> GSHMGFRWKLAHFRYLCQSNALPSHVKINVSRQTLFEDSFQQIMALKPYDLRRRLYVIFRGEEGLDYGGLAREWFFLLSHEVLNPMYCLFEYAGKNNYCLQINPASTINPDHLSYFCFIGRFIAMALFHGKFIDTGFSLPFYKRMLSKKLTIKDLESIDTEFYNSLIWIRDNNIEECGLEMYFSVDMEILGKVTSHDLKLGGSNILVTEENKDEYIGLMTEWRFSRGVQEQTKAFLDGFNEVVPLQWLQYFDEKELEVMLCGMQEVDLADWQRNTVYRHYTRNSKQIIWFWQFVKETDNEVRMRLLQFV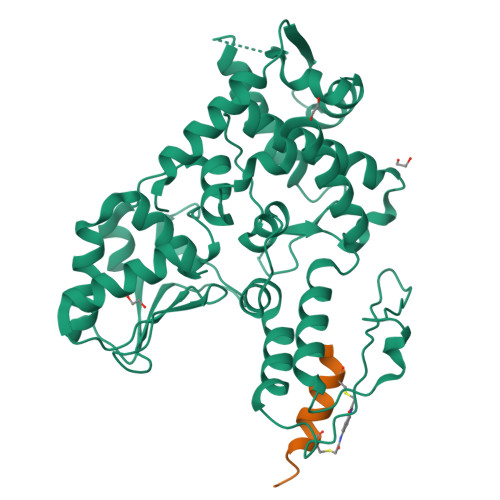TGTCRLPLGGFAELMGSNGPQKFCIEKVGKDTWLPRSHTCFNRLDLPPYKSYEQLKEKLLFAIEETE;> XDPASMRCHRAAHICSVLX Here, we present a strategy for the de novo design of a simplified scaffold of an endo-α-N-acetylgalactosaminidase active site, a glycoside hydrolase from the GH101 enzyme family. Using a combination of trRosetta hallucination, iterative cycles of deep-learning-based structure prediction, and ProteinMPNN sequence design, we designed proteins with 290 amino acids incorporating the active site while reducing the molecular weight by over 100 kDa compared to the initial endo-α-N-acetylgalactosaminidase. Of 11 tested designs, six were expressed as soluble monomers, displaying similar or increased thermostabilities compared to the natural enzyme. Despite lacking detectable enzymatic activity, the experimentally determined crystal structures of a representative design closely matched the design with a root-mean-square deviation of 1.0 Å, with most catalytically important side chains within 2.0 Å.

dEngBF4 crystallized in two different space groups, P212121 (form 1) and P61 (form 2), and the crystal structures of the protein were determined using the molecular replacement method described in Materials and Methods. Form 1 has two protein molecules, 1A and 1B, in the asymmetric unit, whereas for form 2 one protein molecule is present in the asymmetric unit, resulting in three separate structures. All three structures aligned with an RMSD of 1.0 Å or less, revealing a common (β/α)8-barrel organization with an overall fold similar to the hallucinated model. For molecule 1A, more residues were observed in the electron density than in the two other molecules (see above), with the lacking electron density mostly corresponding to residues present within loop regions. Specifically, loop regions ranging from Gly50-Gly65 and Glu210-Val220 were poorly defined or lacked electron density (insert I and II), correlating with regions displaying increased dynamics in the molecular dynamics simulations and low pLDDT confidence score. The dEngBF4 crystal structure (form 1, molecule A) was aligned to the backbone structure of the designed model, revealing a Cα RMSD of 1.0 Å across 191 residues with respect to the OmegaFold model. Notably, the native EngBF active site, which displayed an incomplete (β/α)8-barrel core, was successfully recapitulated in the design, now featuring a fully formed (β/α)8-barrel structure. The specifically restrained catalytic residues exhibited a Cα RMSD of 1.2 Å across 31 atoms relative to the OmegaFold model and 2.0 Å over 34 atoms relative to the EngBF enzyme crystal structure (inserts). Notably, His53 and Asp57 were excluded from this analysis due to their location within a loop region for which electron density was lacking (insert I). Additionally, key catalytic residues, Glu188 and Asp156, corresponding to the catalytic acid/base and nucleophile, respectively, were found to be positioned within 3.4 Å, compared to the 4.2 Å separation observed in EngBF.

>MGEPAKIYINLGVQAPGPFGGGTPEEVAATLDRVKAAAPGIGIIVDLDEGSGVHRDSDHVRLYPEGAGRYTLAEEQAIVDHAKALGAEICYHLNLTVFLPTDPVSEEERAAAKPVWTWTGLHHCIPKEKLLETLLPQKLDELEAAFPGKLDYVYLDRLFDGRCYDLTDEEVRYVLDLIKERGLGIKIESTKYLDTILESGVKVLVDEAVSEKNFDTGKAKVLDPKLFEKYPDLITVEVLYESIETIERALAAGVRNIAIHFGGYGVVSQLDEILDGVRAITENILALASAGSGHHHHHH[2x]>[2x]AIKRIGNHITKSPEDKREYRGLELANGIKVLLISDPTTDKSSAALDVHIGSLSDPPNIAGLSHFLEHMLFLGTKKYPKENEYSQFLSEHAGSSNAFTSGEHTNYYFDVSHEHLEGALDRFAQFFLSPLFDESAKDREVNAVDSEHEKNVMNDAWRLFQLEKATGNPKHPFSKFGTGNKYTLETRPNQEGIDVRQELLKFHSAYYSSNLMAVVVLGRESLDDLTNLVVKLFSEVENKNVPLPEFPEHPFQEEHLKQLYKIVPIKDIRNLYVTFPIPDLQKYYKSNPGHYLGHLIGHEGPG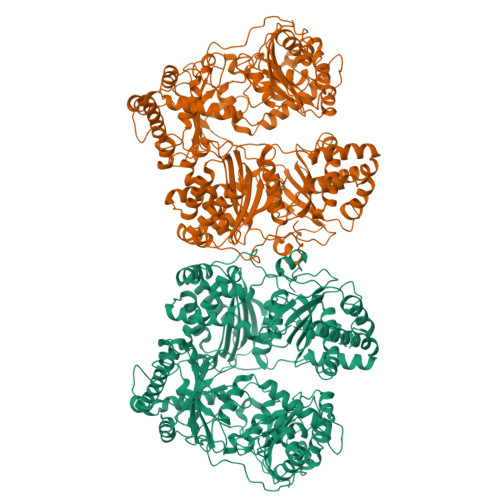SLLSELKSKGWVNTLVGGQKEGARGFMFFIINVDLTEEGLLHVEDIILHMFQYIQKLRAEGPQEWVFQELKDLNAVAFRFKDKERPRGYTSKIAGILHYYPLEEVLTAEYLLEEFRPDLIEMVLDKLRPENVRVAIVSKSFEGKTDRTEEWYGTQYKQEAIPDEVIKKWQNADLNGKFKLPTKNEFIPTNFEILPLEKEATPYPALIKDTAMSKLWFKQDDKFFLPKANLNFEFFSPFAYVDPLHSNMAYLYLELLKDSLNEYAYAAELAGLSYDLQNTIYGMYLSVKGYNDKQPILLKKIIEKMATFEIDEKRFEIIKEAYMRSLNNFRAEQPHQHAMYYLRLLMTEVAWTKDELKEALDDVTLPRLKAFIPQLLSRLHIEALLHGNITKQAALGIMQMVEDTLIEHAHTKPLLPSQLVRYREVQLPDRGWFVYQQRNEVHNNSGIEIYYQTDMQSTSENMFLELFAQIISEPAFNTLRTKEQLGYIVFSGPRRANGIQGLRFIIQSEKPPHYLESRVEAFLITMEKSIEDMTEEAFQKHIQALAIRRLDKPKKLSAESAKYWGEIISQQYNFDRDNTEVAYLKTLTKEDIIKFYKEMLAVDAPRRHKVSVHVLAREMDSCPVVGEFPCQNDINLSQAPALPQPEVIQNMTEFKRGLPLFPLVKPH> HMLSDEQMQIINSLVEAHHKTYDDSYSDFVRFRPPVREGPVTRSASRAASLHSLSDASSDSFNHSPESVDTKLNFSNLLMMYQDSGSPDSSEEDQQSRLSMLPHLADLVSYSIQKVIGFAKMIPGFRDLTAEDQIALLKSSAIEIIMLRSNQSFSLEDMSWSCGGPDFKYCINDVTKAGHTLELLEPLVKFQVGLKKLKLHEEEHVLLMAICLLSPDRPGVQDHVRIEAL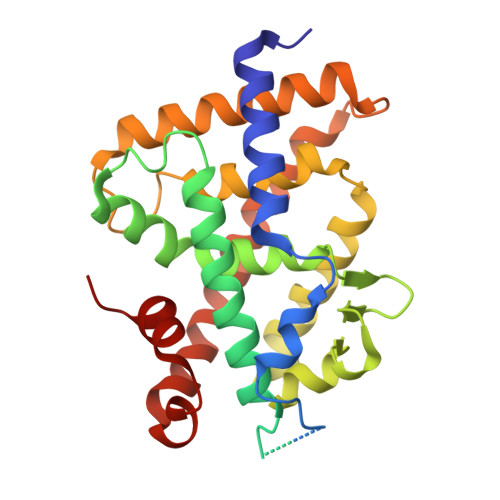QDRLCDVLQAYIRIQHPGGRLLYAKMIQKLADLRSLNEEHSKQYRSLSFQPEHSMQLTPLVLEVFGSEVS> SQQEKPNDNTSNSRDIKNNIQ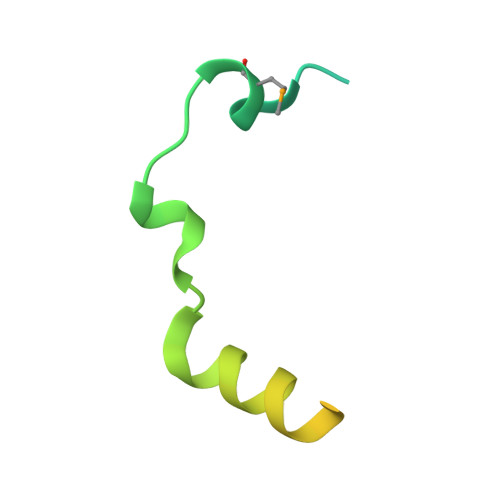FHWKNMTSLSIEECIIPKGQQLILEKESEENTTHGIYLEERKMAQGLHNSVSETPE Black queen cell virus (BQCV) is the etiological agent of a fatal disease of honeybee queen larvae and pupae. The virus belongs to the genus Triatovirus from the family Dicistroviridae, which is part of the order Picornavirales. Viruses from the family Dicistroviridae have nonenveloped icosahedral capsids that protect linear single-stranded positive-sense RNA genomes 8,500 to 10,200 nucleotides in length. The major capsid proteins VP1 to VP3 of dicistroviruses have a jelly roll β-sandwich fold common to capsid proteins of many other viruses and form the capsid shell with pseudo-T= 3 icosahedral symmetry.

The crystal structure of the BQCV virion was determined to a resolution of 3.4 Å. The virion has pseudo-T=3 icosahedral symmetry with 60 copies of each of the viral structural proteins VP1, VP2, and VP3. VP1 subunits form pentamers around the 5-fold axes, whereas VP2 and VP3 subunits constitute alternating heterohexamers around the icosahedral 3-fold axes. A complete model of the major capsid proteins of BQCV could be built except for seven C-terminal residues of VP3. The finger-like protrusions of BQCV reach 34 Å above the virion surface. Each of the protrusions is formed by the C terminus of VP1 and CD loops of VP1 and VP3. However, no density corresponding to VP4 could be identified in the virion structure. SDS gel electrophoresis and mass spectrometry analysis showed that VP4 subunits are present in both native and crystallized BQCV virions. The results show that BQCV virions are infectious even without the structured VP4 subunits, similar to what was shown for TrV. However, BQCV does not harbor such a hydrophobic pocket in the β-barrel of VP1.

> SNSGTEQQNPRGSSLLTDPESITKSDPYNPNISLLISGEVFTNFRNLIKRVNFRKATTLNGKRISDTFDINSLIEAPRLDIAQYVDTETKEAKYGFSYFWSAPTTLNIVAEMYALYRGGVRVKVVTEKGVDFVRATVSPQQTYGSDVAPTTHISTPLAIEQIPIKGVAEFQIPYYAPCLSSSFRANSETFYYSSGRNNLDIATSPPSINRYYAVGAGDDMDFSIFIGTPPCIHASQTAQFTKIKQGKVYDLRYDQYDPFREVQDGTAFLNARSIEDSDLL;> MAEQINENYENKQQLVEQTEITTFENDLIVLEDGPQMEESLPFAFHGQHTDNRQHTVVNFLQRPQVIFDSSWASDVPRNKQFMDSIMIPDDIISFPMFAEKLKGFSSLRATAVITVQFQTQPFQAGRVMLGSFPLPTLNPTRVKFATNHVSRLMLLNHVQCDIAKETEVSLRIPFVSPYNSYDLVSKRFPWAKVVGLVYSPLTTTIPVDFIVYGHFEDVELGCPTSGMLAQ;> SKPLLPIANPTVLRPANTFAITDTNDMSHSLALSNDTNVPFVKALDGSGLDEMSFDYLKKIPQFIQSKFFTTTTKPQEVLFQTKVMPHYFVPGGDVTVAMDKDITRTIWQPSHLAYITSMFKYWTGSLVYTFKFVKTDYHSGRVEVSFHPFSDYTTGTYSDYTYRIIVDLREKSEFSVTIPFISPVPYKRISRPDWDKPYSKYAHASTGTLVLKALTSLKATNTVVSNSVEILIEVNAGDDFNVIAPIENIFFPFSLSPGRKGMVAQ> SPRLP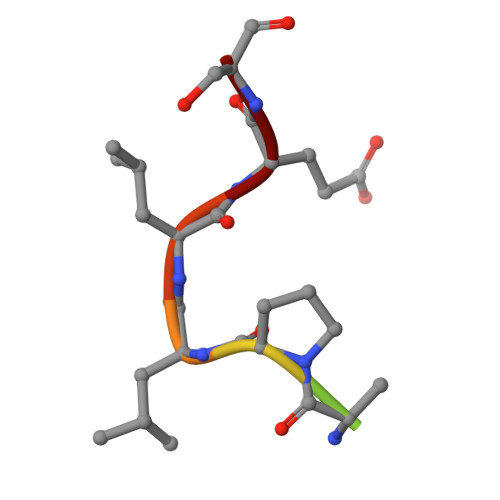LLES>[6x]MADFKFEPMRSLIYVDCVSEDYRPKLQRWIYKVHIPDSISQFEPYVTKYAFYPSFPIPPQGDRFGYARMQLTEHHWLVSDLDPRLEIKAIAETFPMDVLVWQGQIPAAAHTDAQIDSDGDAGNAARKSNNAEGNPFIFAFLPMWWEKDLKGKGRTIEDGANYRFNMTIGFPEGVDKAEGEKWLFEKVVPILQAAPECTRVLASAVKKDINGCVMDWVLEIWFENQSGWYKVMVDDMKALEKPSWAQQDAFPFLKPYHNVCSAAVADYTPSNNLANYRGYITMR

The bacterial chalcone isomerase (CHI) from Eubacterium ramulus catalyses the first step in a flavanone-degradation pathway by a reverse Michael addition. The overall fold and the constitution of the active site of the enzyme completely differ from the well-characterised chalcone isomerase of plants. The quaternary structure is a hexamer with D3 symmetry (trimer of dimers). The tertiary structure of bacterial CHI (polypeptide with 282 amino-acid residues) is separated into a catalytic- and solvent-exposed domain, both with ferredoxin-like folds, completely different to that of the plant CHI, suggesting that the enzyme activities convergently evolved from different ancestor proteins.

Crystals of native CHI and CHI_H33A were soaked in the substrate (2R,3R)-dihydroquercetin ((+)-taxifolin, Protein Data Bank (PDB) three-letter code DQH) and X-ray diffraction data were collected. The electron-density maps of native CHI soaked with DQH show a complicated disorder in the active sites. Clearly, this structure analysis is not the doubtless identification of a distinct molecule in the active site, but more of a snapshot of the enzyme at work. The C6-C3-C6 framework cannot be clearly identified as one of the possible substrate or product molecules. We see two electron density bubbles at the positions of the A and B ring, but a gap for the connection. This can be interpreted as a superposition of substrate, intermediates, and product caused by equilibria on the reaction pathway. The observed electron density might be caused by alternative substrate and product binding in the active sites, but additionally, the reaction intermediates, the chalcone and the di-keto-tautomer, should be considered. Initial crystallographic refinement was tested with each of the four molecules of the reaction pathway. According to refinement statistics and electron density maps, the final model building and refinement was performed with the taxifolin chalcone, which marginally turned out as the best. No additional substrate binding in the active site was observed.Bacterial transcription termination factor, ρ, is a hexameric, NTP-dependent 5’–3’ RNA translocase and helicase. A ρ monomer contains N-terminal (NTD) and C-terminal (CTD) domains connected by a flexible linker. The NTD comprises an N-terminal three-helix bundle and a five-stranded β-barrel, the OB-fold, that forms a primary RNA-binding site (PBS); the PBSes are located around one outer rim of the ρ hexamer. The CTDs jointly form a secondary RNA-binding site (SBS) at the center of the ρ hexamer.

We subjected SEC fractions corresponding to ρ-Rof complexes to cryoEM/SPA in the absence and presence of the transition state analog, ADP-BeF3. Multi-particle 3D refinement with ~600,000 particle images yielded two cryoEM reconstructions for each sample, corresponding to two ρ-Rof assemblies. In the first assembly, ρ forms an open hexameric ring (ρA-ρF) bound by five Rof molecules (Rofa-Rofe), while the second assembly represents a ρ pentamer (ρA-ρE) bound by four Rof molecules (Rofa-Rofd). In the presence of ADP-BeF3, we obtained a ~1:1 (ρ6-Rof5:ρ5-Rof4) distribution between the two classes, whereas in the absence of the nucleotide, the equilibrium was shifted towards the lower oligomeric assembly (ρ6-Rof5:ρ5-Rof4 ~ 1:3). The reconstructions do not reveal differences in the ρ-Rof interfaces, irrespective of oligomeric state or bound nucleotide. Rof molecules are bound between protomers ρA-ρB, ρB-ρC, etc., but not preceding or following the terminal ρ subunits, ρA and ρF. In addition, loopβ3-β4 of Rof contacts the N-terminal three-helix bundle of the adjacent ρ protomer, presumably explaining why Rof binding is only observed between neighboring ρ subunits but not at the terminal subunits of the open ring. Thus, Rof bound between two neighboring NTDs of open ρ may stabilize their relative positions, and thus the open-ring conformation.

>[6x]MNLTELKNTPVSELITLGENMGLENLARMRKQDIIFAILKQHAKSGEDIFGDGVLEILQDGFGFLRSADSSYLAGPDDIYVSPSQIRRFNLRTGDTISGKIRPPKEGERYFALLKVNEVNFDKPENARNKILFENLTPLHANSRLRMERGNGSTEDLTARVLDLASPIGRGQRGLIVAPPKAGKTMLLQNIAQSIAYNHPDCVLMVLLIDERPEEVTEMQRLVKGEVVASTFDEPASRHVQVAEMVIEKAKRLVEHKKDVIILLDSITRLARAYNTVVPASGKVLTGGVDANALHRPKRFFGAARNVEEGGSLTIIATALIDTGSKMDEVIYEEFKGTGNMELHLSRKIAEKRVFPAIDYNRSGTRKEELLTTQEELQKMWILRKIIHPMGEIDAMEFLINKLAMTKTNDDFFEMMKRS;>AMGNDTYQPINCDDYDNLELACQHHLMLTLELKDGEKLQAKASDLVSRKNVEYLVVEAAGETRELRLDKITSFSHPEIGTVVVSES[5x]~{N}-oxidanyl-4-[(5-thiophen-2-yl-1,2,3,4-tetrazol-1-yl)methyl]benzamide | C13 H11 N5 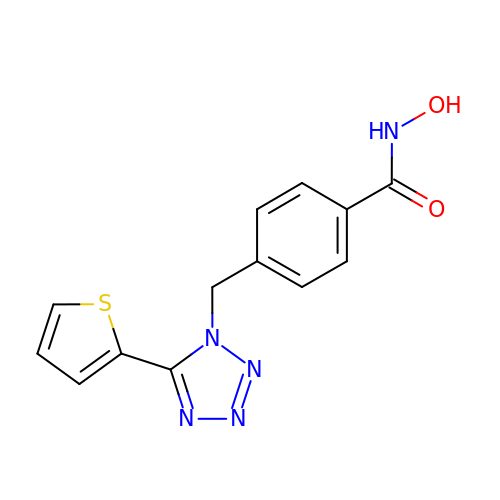O2 S | UFUGFWWXDWPEQE-UHFFFAOYSA-N>MYGLVNKAIQDMISKHHGEDTWEAIKQKAGLEDIDFFVGMEAYSDDVTYHLVGAASEVL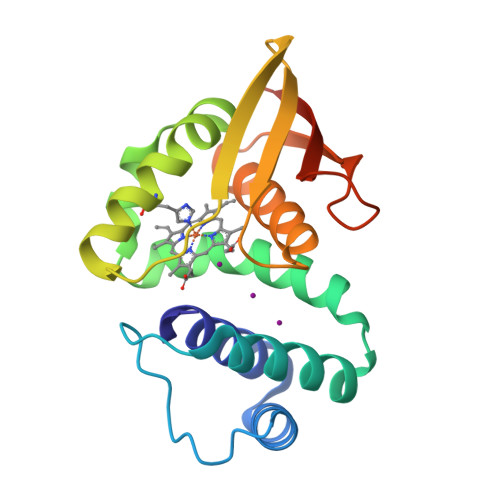GKPAEELLIAFGEYWVTYTSEEGYGELLASAGDSLPEFMENLDNLHARVGLSFPQLRPPAFECQHTSSKSMELHYQSTRCGLAPMVLGLLHGLGKRFQTKVEVTQTAFRETGEDHDIFSIKYEDSNLYDD[2x]>[2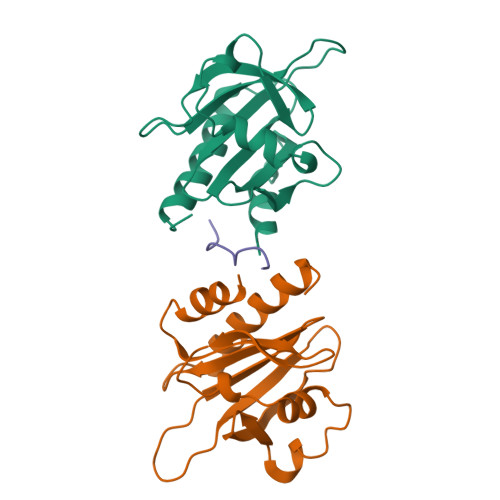x]GWNAYIDNLMADGTCQDAAIVGYKDSPSVWAAVPGKTFVNITPAEVGVLVGKDRSSFYVNGLTLGGQKCSVIRDSLLQDGEFSMDLRTKSTGGAPTFNVTVTKTDKTLVLLMGKEGVHGGLINKKCYEMASHLRRSQY;> PPPPPPPPPP> SKPRNQNQVMPYQNVPGWGYSLYKGIDMSVPLAYDPNNELGDLRDVFPSAVDEMAIGYVCGNPAIKHVLTWSTTDVVQNPISNGDDWGGVIPVGMPCYSKTIRAVKGATS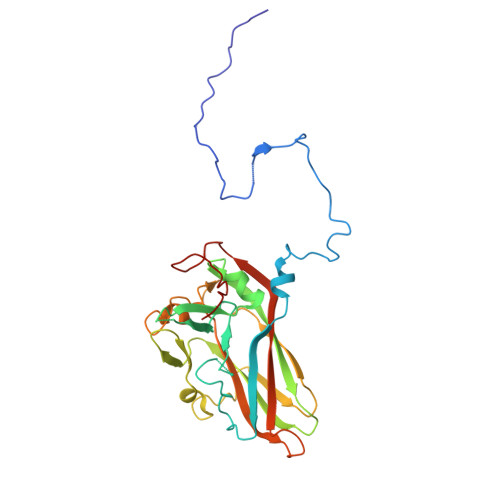TSKTEVMDPAPCEYVANLFSYWRATMCYRITVVKTAFHTGRLEIFFEPGSIPTVRTADNLGPDQTQLNGTIAPSDNNYKYILDLTNDTEVTIKVPYVSNKMFMKTVGIYGAHDEDNWNFDESFTGFLCIRPITKLMAPDTVSQKVSIVVWKWAEDVVVVEPKPLTSGPTQVYNPPAVA> MGHHHHHHSRSVRHIAIPAHRGLITDRNGEPLAVSTPVTTLWANPKELMTAKERWPQLAAALGQDTKLFADRIEQNAEREFIYLVRGLTPEQGEGVIALKVPGVYSIEEFRRFYPAGEVVAHAVGFTDVDDRGREGIELAFDEWLAGVPGKRQVLKD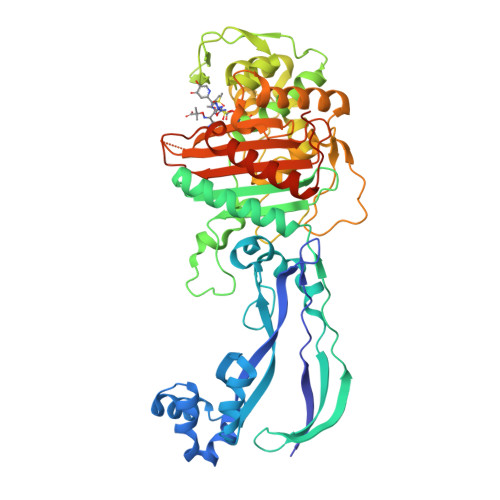RRGRVIKDVQVTKNAKPGKTLALSIDLRLQYLAHRELRNALLENGAKAGSLVIMDVKTGEILAMTNQPTYNPNNRRNLQPAAMRNRAMIDVFEPGSTVKPFSMSAALASGRWKPSDIVDVYPGTLQIGRYTIRDVSRNSRQLDLTGILIKSSNVGISKIAFDIGAESIYSVMQQVGLGQDTGLGFPGERVGNLPNHRKWPKAETATLAYGYGLSVTAIQLAHAYAALANDGKSVPLSMTRVDRVPDGVQVISPEVASTVQGMLQQVVEAQGGVFRAQVPGYHAAGKSGTARKVSVGTKGYRENAYRSLFAGFAPATDPRIAMVVVIDEPSKAGYFGGLVSAPVFSKVMAGALRLMNVPPDNLPTATEQQQVNAAPAKGGRG>[2x]MSAAADRLNLTSGHLNAGRKRSSSSVSLKAAEKPFKVTVIGSGNWGTTIAKVVAENCKG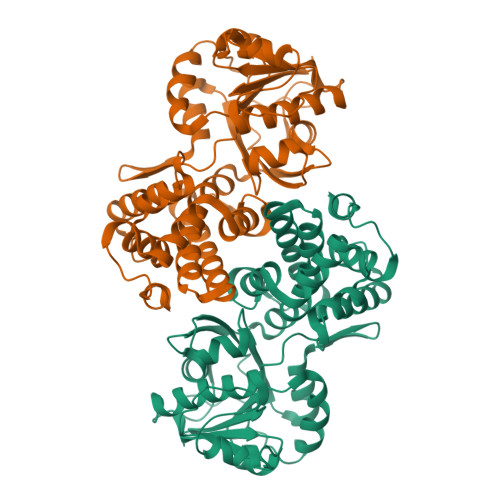YPEVFAPIVQMWVFEEEINGEKLTEIINTRHQNVKYLPGITLPDNLVANPDLIDSVKDVDIIVFNIPHQFLPRICSQLKGHVDSHVRAISCLKGFEVGAKGVQLLSSYITEELGIQCGALSGANIATEVAQEHWSETTVAYHIPKDFRGEGKDVDHKVLKALFHRPYFHVSVIEDVAGISICGALKNVVALGCGFVEGLGWGNNASAAIQRVGLGEIIRFGQMFFPESREETYYQESAGVADLITTCAGGRNVKVARLMATSGKDAWECEKELLNGQSAQGLITCKEVHEWLETCGSVEDFPLFEAVYQIVYNNYPMKNLPDMIEELDLHED> SEAEARPTNFIRQIIDEDLASGKHTTVHTRFPPEPNGYLHIGHAKSICLNFGIAQDYKGQCNLRFDDTNPVKEDIEYVESIKNDVEWLGFHWSGNVRYSSDYFDQLHAYAIELINKGLAYVDELTPEQTREYRGTLTQPGKNSPYRDRSVEENLALFEKMRAGGFEEGKACLRAKIDMASPFIVMRDPVLYRIKFAEHHQTGNKWCIYPMYDFTHCISDALEGITHSLCTLE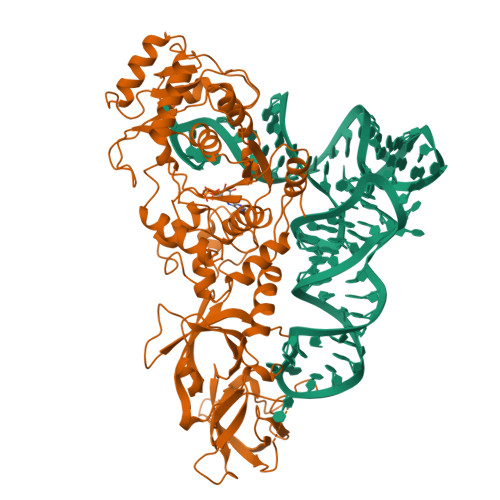FQDNRRLYDWVLDNITIPVHPRQYEFSRLNLEYTVMSKRKLNLLVTDKHVEGWDDPRMPTISGLRRRGYTAASIREFCKRIGVTKQDNTIEMASLESCIREDLNENAPRAMAVIDPVKLVIENYQGEGEMVTMPNHPNKPEMGSRQVPFSGEIWIDRADFREEANKQYKRLVLGKEVRLRNAYVIKAERVEKDAEGNITTIFCTYDADTLSKDPADGRKVKGVIHWVSAAHALPVEIRLYDRLFSVPNPGAADDFLSVINPESLVIKQGFAEPSLKDAVAGKAFQFEREGYFCLDSRHSTAEKPVFNRTVGLRDTWAKVGE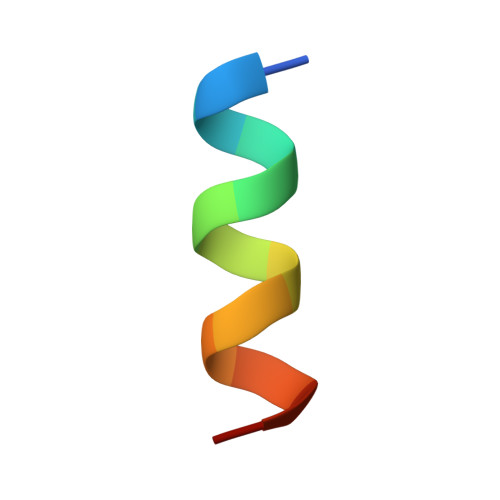> TSGSNELLSILHRK>[2x]QLRYSVPEEQSPGALVGNVARALGLELRRLGPGCLRINHLGAPSPRYLELDLTNGALFVNERIDREALCEQRPRCLLSLEVLAHNPVAVSAIEVEILDINDNSPRFPRPDYQLQVSESVAPGARFHIESAQDPDVGANSVQTYELSPSEHFELDLKPLQENSKVLELVLRKGLDREQTALHYLVLTAVDGGIPARSGTAQIAVRVLDT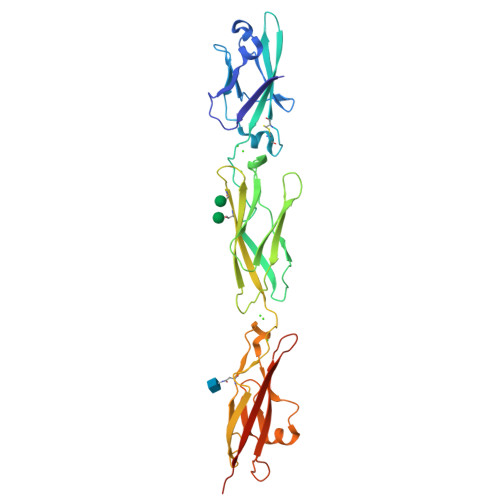NDNSPAFDQSTYRVQLREDAPPGTLVVKLNASDPDEGSNGELRYSLSSYTSDRERQLFSIDVTTGEVRVSGTLDYEESSSYQIYVQATDRGPVPMAGHCKVLVDIIDVNDHHHHHHHH>NLQNIIYNPVIPFVGTIPDQLDPGTLIVIRGHVPSDADRFQVDLQNGSSMKPRADVAFHFNPRFKRAGCIVCNTLINEKWGREEITYDTPFKREKSFEIVIMVLKDKFQVAVNGKHTLLYGHRIGPEKIDTLGIYGKVNIHSIGF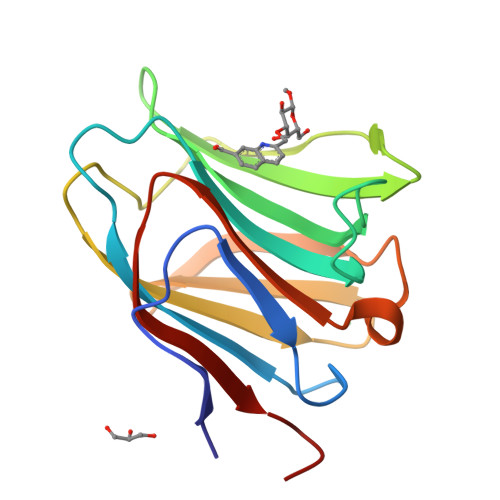SFSSD[2x]>MNNHFKCIGIVGHPRHPTALTTHEMLYRWLCDQGYEVIVEQQIAHELQLKNVPTGTLAEIGQQADLAVVVGGDGNMLGAARTLARYDINVIGINRGNLGFLTDLDPDNALQQLSDVLEGRYISEKRFLLEAQVCQQDRQKRISTAINE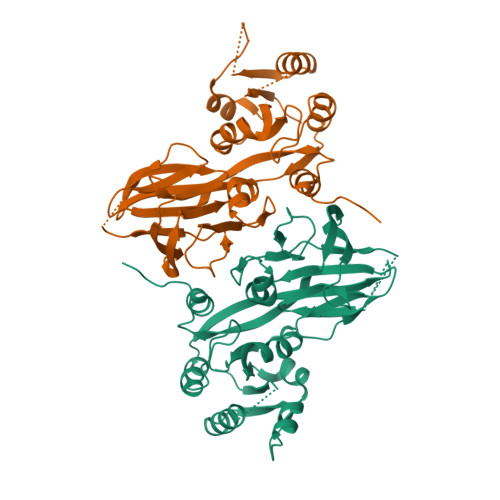VVLHPGKVAHMIEFEVYIDETFAFSQRSDGLIISTPTGSTAYSLSAGGPILTPSLDAITLVPMFPHTLSARPLVINSSSTIRLRFSHRRSDLEISCDSQIALPIQEGEDVLIRRCDYHLNLIHPKDYSYFNTLSTKLGWSKKLF[4x]> GAHMSGRMTDDKDVLRDVWFGRIPTCFTLYQDEITEREAEPYYLLLPRVS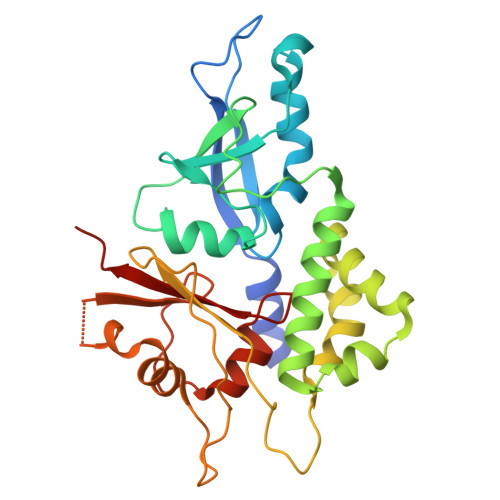YLTLVTDKVKKHFQKVMRQEDISEIWFEYEGTPLKWHYPIGLLFDLLASSSALPWNITVHFKSFPEKDLLHCPSKDAIEAHFMSCMKEADALKHKSQVINEMQKKDHKQLWMGLQNDRFDQFWAINRKLMEYPAEENGFRYIPFRIYQTTTERPFIQKLFRPVAADGQLHTLGDLLKEVCPSAIDPEDGEKKNQVMIHGIEPMLETPLQWLSEHLSYPDNFLHISIIPQPTD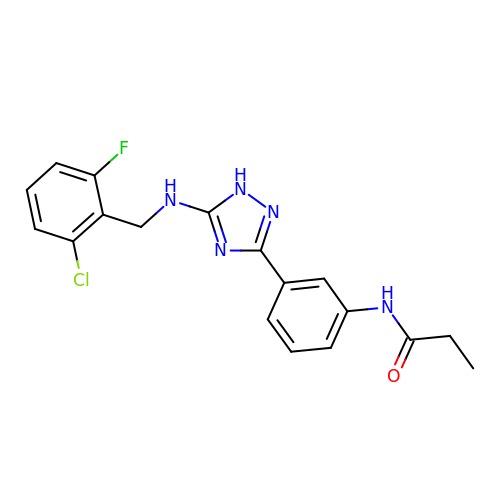N-[3-(5-{[(2-chloro-6-fluorophenyl)methyl]amino}-1H-1,2,4-triazol-3-yl)phenyl]propanamide | C18 H17 Cl F N5 O | RBMCVMVCNBYBCI-UHFFFAOYSA-N COPROPORPHYRINOGEN I | C36 H44 N4 O8 | 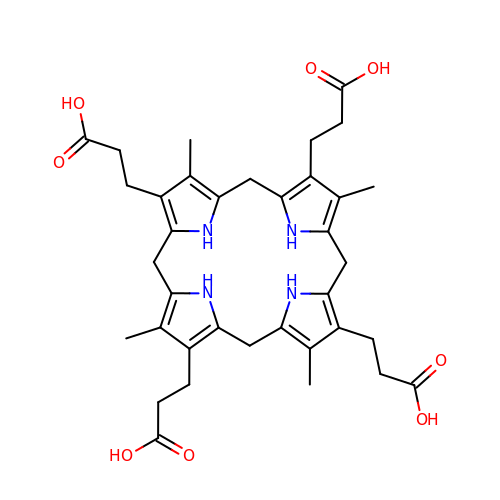WIUGGJKHYQIGNH-UHFFFAOYSA-N>NEVTLLDSRSVQGELGWIASPLEGGWEEVSIMDEKNTPIRTYQVCNVMEPSQNNWLRTDWITREGAQRVYIEIKFTLRDCNSLPGVMGTCKETFNLYYYESDNDKERFIRENQFVKIDT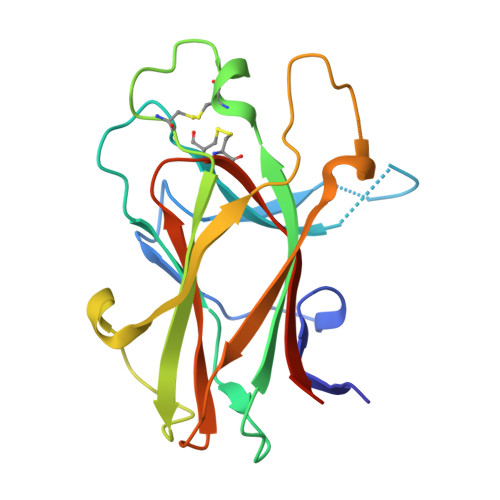IAADESFTQVDIGDRIMKLNTEIRDVGPLSKKGFYLAFQDVGACIALVSVRVFYKKAPLTVR[2x]>MRGSHHHHHHGMASMPLHHLTRFPRLEFIGAPTPLEYLPRLSDYLGREIYIKRDDVTPIAMGGNKLRKLEFLVADALREGADTLITAGAIQSNHVRQTAAVAAKLGLHCVALLENPIGTTAENYLTNG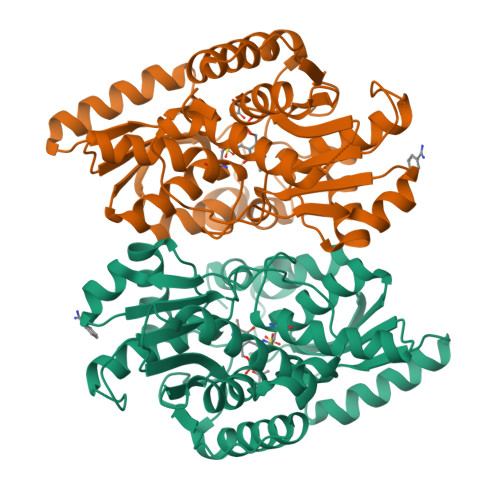NRLLLDLFNTQIEMCDALTDPDAQLQTLATRIEAQGFRPYVIPVGGSSALGAMGYVESALEIAQQCEEVVGLSSVVVASGSAGTHAGLAVGLEHLMPDVELIGVTVSRSVAEQKPKVIALQQAIAGQLALTATADIHLWDDYFAPGYGVPNDAGMEAVKLLASLEGVLLDPVYTGKAMAGLIDGISQKRFNDDGPILFIHTGGAPALFAYHPHV[4x]> EPAENSDFYLPGDYLLGGLFSLHANMKGIVHLNFLQVPMCKEYEVKVIGYNLMQAMRFAVEEINNDSSLLPGVLLGYEIVDVCYISNNVQPVLYFLAHEDNLLPIQEDYSNYSSRVVAVIGPDNSESVMTVANFLSLFLLPQITYSAISDELRDKVRFPALLRTTPSADHHIEAMVQLMLHFRWNWIIVLVSNDTYGRDNGQLLGERVARRDICIAFQETLPTLQPNQNMTSEERQRLVTIVDKLQQSTARVVVVFSPDLTLYHFFNEVLRQNFTGAVWIASESWAIDPVLHNLTELRHLGTFLGITIQSVPIPGFSEFREWGPQAGPPPLSRTSQSYTCNQECDNCLNATLSFNTILRLSGERVVYSVYSAVYAVAHALHSLLGCDKSTCTKRVVYPWQLLEEIWKVNFTLLDHQIFFDPQGDVALHLEIVQWQWDRSQNPFQSVASYYPLQRQLKNIQDISWHTINNTIPMSMCSKRCQSGQKKKPVGIHVCCFECIDCLPGTFLNHTEDEYECQACPNNEWSYQSETSCFKRQLVFLEWHEAPTIAVALLAALGFLSTLAILVIFWRHFQTPIVRSAGGPMCFLMLTLLLVAYMVVPVYVGPPKVSTCLCRQALFPLCFTICISCIAVRSFQIVCAFKMASRFPRAYSYWVRYQGPYVSMAFITVLKMVIVVIGMLATGLSPTTRTDPDDPKITIVSCN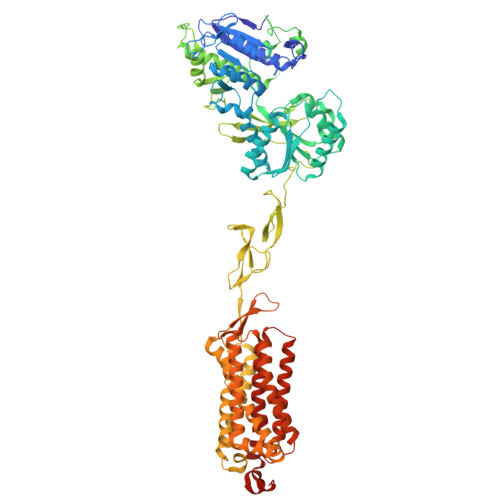PNYRNSLLFNTSLDLLLSVVGFSFAYMGKELPTNYNEAKFITLSMTFYFTSSVSLCTFMSAYSGVLVTIVDLLVTVLNLLAISLGYFGPKCYMILFYPERNTPAYFNSMIQGYTMRRD> MGSSHHHH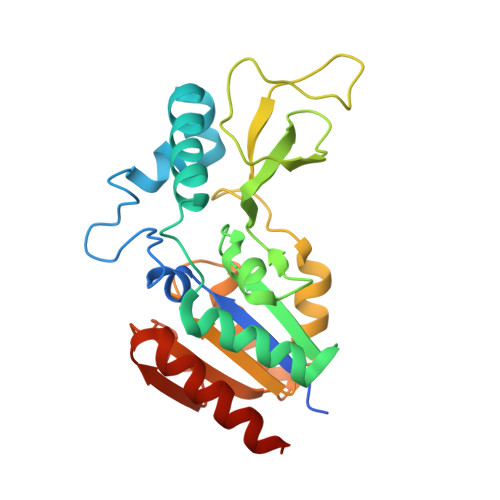HHSQDPKPRVLVLTGAGISAESGIRTFRAADGLWEEHRVEDVATPEGFDRDPELVQAFYNARRRQLQQPEIQPNAAHLALAKLQDALGDRFLLVTQNIDNLHERAGNTNVIHMHGELLKVRCSQSGQVLDWTGDVTPEDKCHCCQFPAPLRPHVVWFGEMPLGMDEIYMALSMADIFIAIGTSGHVYPAAGFVHEAKLHGAHTVELNLEPSQVGNEFAEKYYGPASQVVPEFVEKLLKGLKAGSIA>EKPKLHITMFPWVAIGHITPFIHLANELAKRGHSISILIPKKAHTQLGHNNLYPDLIKFHIVTVPHVEGLPAGAETASDIDITAKNPLAIAFDAMYEQVETLLYGLKPDIVFYDFADWIPKLAAQIGFKTVCYNVICASCMAIGIVPARHIPKDRPLTEEELMTPPEGYPSSTVVLRGQEARTLSFIGMDYGATKFDVRITAAMQGCDAIGIRTCRELEGPMCDYLSAQYNKPVFLSGPVLPESPKGPLEEKWEKWLNKFEPKSVVYCAFGSQMILQKNQFQELVLGFEMTGLPFFVALSKPHGADSIEEALPEGFLERVGDRGVVHGGWVQQTQILNHQSVGCFVSHCGFGSMWESLLS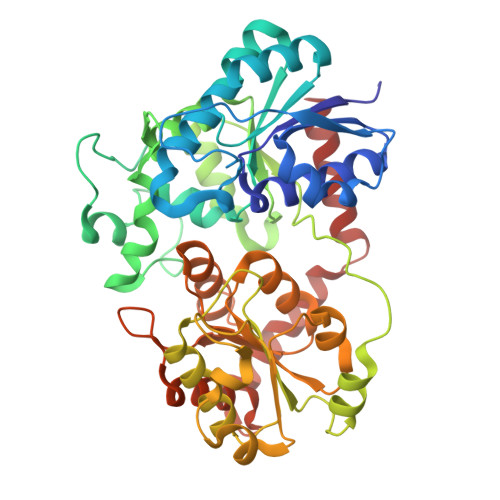DSQIVLVPRLADQILNTRLLAEELKVAVEVERGDMGWFSKEDLCKAIKSVMDEESEVGKLVKKNHAKWRETLVSPGYMDNYLEDFIQQLYG[2x]>[2x]MSPKLPQHGTVGVRTPLVDGVEKVTGKAKYTADIAAPDALVGRILRSPHAHARILAIDTSAAEALEGVIAVCTGAETPVPFGVLPIAENEYPLARDKVRYRGDPVAAVAAIDEVTAEKALALIKVDYEVLPAYMTPKAAMKAGAIALHDDKPNNILREVHAEFGDVAAAFAEADLIREKTYTFAEVNHVHMELNATLAEYDPVRDMLTLNTTTQVPYYVHLKVAACLQMDSARIRVIKPFLGGGFGARTEALHFEIIAGLLARKAKGTVRLLQTREETFIAHRGRPWTEVKMKIGLKKDGKIAALALEATQAGGAYAGYGIITILYTGALMHGLYHIPAIKHDAWRVYTNTPPCGAMRGHGTVDTRAAFEALLTEMGEELGIDSLKIRQINMLPQIPYVTMYAQRVMSYGVPECLEKVKAASGWEERKGKLPKGRGLGIALSHFVSGTSTPKHWTGEPHATVNLKLDFDGGITLLTGAADIGQGSNTMASQVAAEVLGVRLSRIRVISADSALTPKDNGSYSSRVTFMVGNASISAAEELKGVLVKAAAKKLDAREEDIEVIDEMFMVSGSQDPGLSFQEVVKAAMVDSGTITVKGTYTCPTEFQGDKKIRGSAIGATMGFCYAAQVVEASVDEITGKVTAHKVWVAVDVGKALNPLAVEGQTQGGVWMGMGQALSEETVYDNGRMVHGNILDYRVPTIVESPDIEVIIVESMDPNGPFGAKEASEGMLAGFLPAIHEAVYEAVGVRATDFPLSPDRITELLDAKEAAA;>[2x]MNILTDFRTHRPATLADAVNALAAEATLPLGAGTDLLPNLRRGLGHPAALVDLTGIDGLATISTLADGSLRIGAGATLEAIAEHDAIRTTWPALAQAAESVAGPTHRAAATLGGNLCQDTRCTFYNQSEWWRSGNGYCLKYKGDKCHVIVKSDRCYATYHGDVAPALMVLDARAEIVGPAGKRTVPVAQLFRESG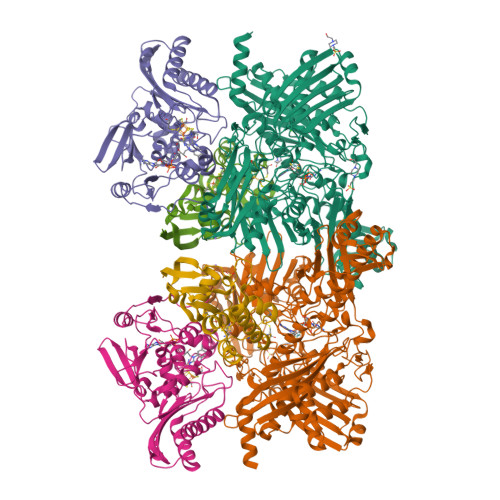AEHLTLEKGELLAAIEVPPTGAWSAAYSKVRIRDAVDFPLAGVAAALQRDGDRIAGLRVAITGSNSAPLMVPVDALLGGNWDDAAAETLAQLVRKTSNVLRTTITGVKYRRRVLLAISRKVVDQLWEAR;>[2x]MKNILRLTLNGRAREDLVPDNMLLLDYLRETVGLTGTKQGCDGGECGACTVLVDDRPRLACSTLAHQVAGKKVETVESLATQGTLSKLQAAFHEKLGTQCGFCTPGMIMASEALLRKNPSPSRDEIKAALAGNLCRCTGYVKIIKSVETAAAARLCEEGAR> MTLAFGDWIVHRRWYAGRSRELVSAEPAVVTPLRDDLDHILLDVTYTDGTVERYQLVVRWADSPVAGFGEAATIGTALGPQGERIAYDALFDPDAARHLLRLVDASATVADLRFTREPGATLPLYAPPKVSSAEQSNTSVIFGKDAMLKVFRRVTPGINPDIELNRVLAQAGNRHVARLLGSFETSWAGPGTDRCALGMVTAFAANSAEGWDMATASAREMFADVVGSDFADESYRLGNAVASVHATLAEALGTSTEPFPVDTVLARLQSAARSAPELAGRAAAVEERYRRLDGRAITVQRVHGDLHLG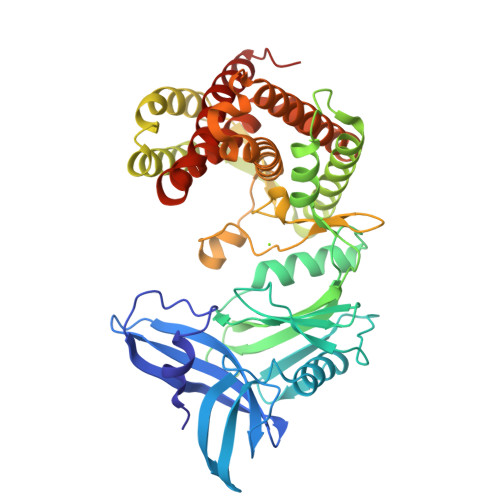QVLRTPDDWLLIDFEGEPGQPLDERRRPDSPLRDVAGVLRSFEYAAYQKLVELAPEQDADGRLADRARNWVDRNSAAFCAGYAAVAGDDPRRDGDVLAAYELDKAVYEAAYEARFRPSWLPIPMRSIDRILGKLAAALEHHHHHH>MSLRSKRSNVVGLIVSDIENVFFAEVASGVESEARHKGYSVLLANTAEDIVREREAVG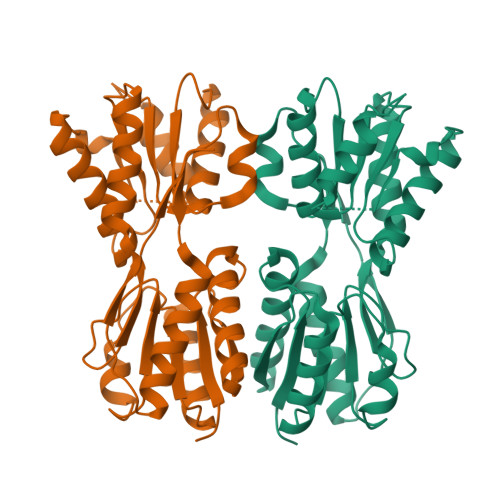QFFERRVDGLILAPSEGEHDYLRTELPKTFPIVAVNRELRIPGCGAVLSENVRGARTAVEYLIARGHTRIGAIVGSAGLMTSRERLKGFRAAMSAAGLPVRQEWIAAGGVRADNGRDGAIKVLTGADRPTALLTSSHRITEGAMQALNVLGLRYGPDVEIVSFDNLPWMAFLDPPLPVVEQPTRRIGQEAMRMLIHMIEGTGNATEMRLQTRFVTHVGQDLSVEAEGHHHHHH[6x]>[2x]APQQINDIVHRTITPLIEQQKIPGMAVAVIYQGKPYYFTWGYADIAKKQPVTQQTLFELGSVSKTFTGVLGGDAIARGEIKLSDPTTKYWPELTAKQWNGITLLHLATYTAGGLPLQVPDEVKSSSDLLRFYQNWQPAWAPGTQRLYANSSIGLFGALAVKPSGLSFEQAMQTRVFQPLKLNHTWINVPPAEEKNYAWGYREGK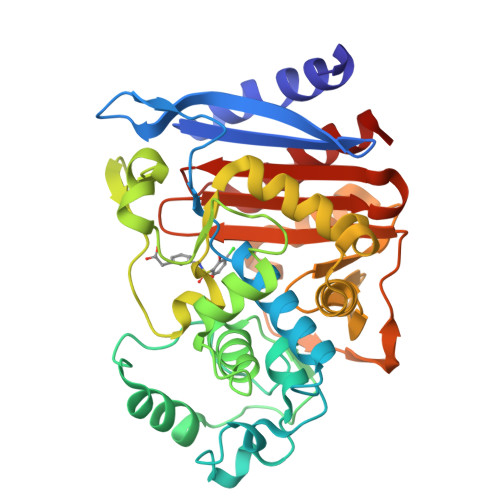AVHVSPGALDAEAYGVKSTIEDMARWVQSNLKPLDINEKTLQQGIQLAQSRYWQTGDMYQGLGWEMLDWPVNPDSIINGSDNKIALAARPVKAITPPTPAVRASWVHKTGATGGFGSYVAFIPEKELGIVMLANKNYPNPARVDAAWQILNALQ>[2x]MTTSESPDAYTESFGAHTIVKPAGPPRVGQPSWNPQRASSMPVNRYRPFAEEVEPIRLRNRTWPDRVIDRAPLWCAVDLRDGNQALIDPMSPARKRRMFDLLVRMGYKEIEVGFPSASQTDFDFVREIIEQGAIPDDVTIQVLTQCRPELIERTFQACSGAPRAIVHFYNSTSILQRRVVFRANRAEVQAIATDGARKCVEQAAKYPGTQWRFEYSPESYTGTELEYAKQVCDAVGEVIAPTP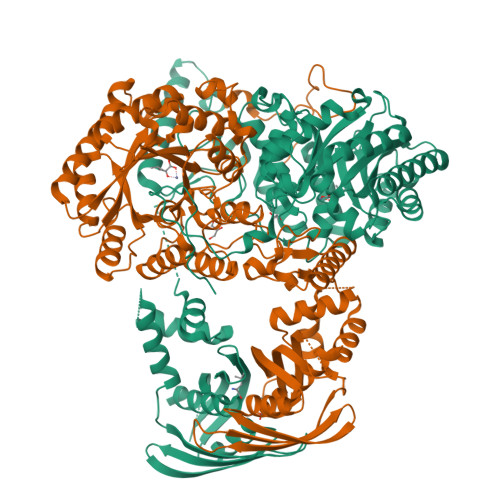ERPIIFNLPATVEMTTPNVYADSIEWMSRNLANRESVILSLHPHNDRGTAVAAAELGFAAGADRIEGCLFGNGERTGNVCLVTLGLNLFSRGVDPQIDFSNIDEIRRTVEYCNQLPVHERHPYGGDLVYTAFSGSHQDAINKGLDAMKLDADAADCDVDDMLWQVPYLPIDPRDVGRTYEAVIRVNSQSGKGGVAYIMKTDHGLSLPRRLQIEFSQVIQKIAEGTAGEGGEVSPKEMWDAFAEEYLAPVRPLERIRQHVDAADDDGGTTSITATVKINGVETEISGSGNGPLAAFVHALADVGFDVAVLDYYEHAMSAGDDAQAAAYVEASVTIASPAQPGEAGRHASDPVTIASPAQPGEAGRHASDPVTSKTVWGVGIAPSITTASLRAVVSAVNRAAR> FVVEKNNLKVTSPDSIKGIYECAIGNFGVPQYGGTLVGTVVYPKSNQKACKSYSDFDISFKSKPGRLPTFVLIDRGDCYFTLKAWIAQQAGAAAILVADSKAEPLITMDTPEEDKSDADYLQNITIPSALITKTLGDSIKSALSGGDMVNMKLDWTESVPHPDERVEYELWTNSNDECGKKCDTQIEFLKNFKGAAQILEKGGHTQFTPHYITWYCPEAFTLSKQCKSQCINHGRYCAPDPEQDFTKGYDGKDVVVQNLRQACVYRVMNDTGKPWVWWDYVTDFAIRCPMKEKKYTKECADGIIKSLGIDLKKVDKCIGDPEADVENPVLKAEQESQIGKGSRGDVTILPTLVVNNRQYRGKLEKGAVLKAMCSGFQESTEPAICLTEDLETNECLENNGGCWQDKAANITACRDTFRGRLCECPTVQGVKFVGDGYTHCKASGALHCGINNGGCWRESRGGFTYSACVDDHSKDCKCPLGFKGDGVKNCEDVDECKEKTVCQCPECKCKNTWGSYECSCSNGLLYMREHDTCIGSGKVGTTKLSWSFLWILIIGVGVAGLS

The vacuolar sorting receptors (VSRs) are specific to plants and are responsible for sorting and transporting particular proteins from the trans-Golgi network to the vacuole. This process is critically important for various cellular functions, including storing nutrients during seed development. VSRs are type-I transmembrane proteins with ~ 600 amino acids (80 kDa without the N-terminal signaling peptide).

Herein, we report a crystal structure of full-length VSR1 luminal domain from Arabidopsis thaliana (AtVSR1). The structural model starts at Phe21 and ends at Ala465 and the overall structure is separated into three distinct domains: the PA domain (Phe21-Trp175), the thioredoxin (TRX) domain (Val186-Phe396), and the EGF-like domain (Glu409-Ala462). The resolved structure had disordered regions at the C-terminus, where density could not be uniquely traced for proper model building after the first EGF-like domain. At the beginning of the refinement, a clear electron density attached to the sidechain of Asn289 in the central domain was observed and assigned as two N-acetylglucosamine (GlcNAc). The PA and the TRX domains are connected by a 7-residue linker with no significant interaction between them. Although there is no direct interaction between the intramolecular PA and TRX domains, the two domains display extensive interactions with those domains of two neighboring molecules related by a crystallographic threefold symmetry, forming a cyclical domain-swapping. PDBePISA analysis of the crystallographic intermolecular interaction between the PA and the TRX domains reveals that the interface score is 1.0, indicating that AtVSR1 is highly likely to form a trimer in solution. The interaction between the TRX and EGF-like domains is held by multiple H-bond interactions. The two additional EGF-like domains that are tandemly located at the C-terminus are not visible in the crystal structure, indicating their high flexibility. However, our crystal structure shows that the AtVSR1 has an extended conformation with significant dynamic flexibility of the EGF-like domains.>[2x]QDADKLPHTKVTLVAPPQVHPHEQATKSGPKVVEFTMTIEEKKMVIDDKGTTLQAMTFNGSMPGPTLVVHEGDYVQLTLVNPATNAMPHNVDFHGATGALGGAKLTNVNPGEQATLRFKADRSGTFVYHCAPEGMVPWHVVSGMSGTLMVLPRDGLKDPQGKPLH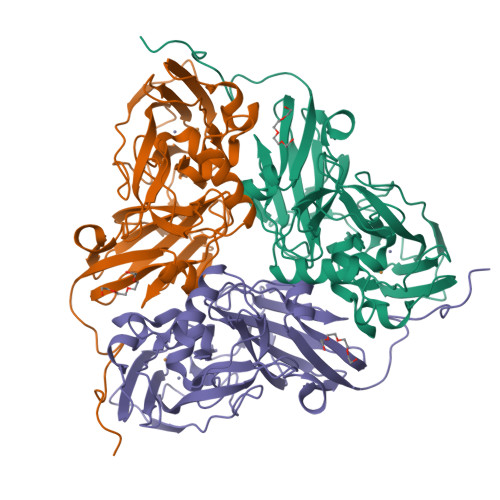YDRAYTIGEFDLYIPKGPDGKYKDYATLAESYGDTVQVMRTLTPSHIVFNGKVGALTGANALTAKVGETVLLIHSQANRDTRPHLIGGHGDWVWETGKFANPPQRDLETWFIRGGSAGAALYTFKQPGVYAYLNHNLIEAFELGAAGHIKVEGKWNDDLMKQIKAPAPIPR>[2x]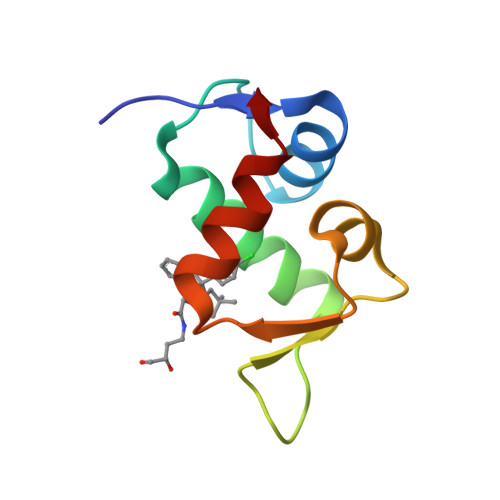EKLVQPTPLLLSLLKSAGAQKETFTMKEVLYHLGQYIMAKQLYDEKQQHIVHCSNDPLGELFGVQEFSVKEHRRIYAMISRNLVS> MSGGSPAEREAGRIVVRGDVAIAEAVVRKVGEVAGKEVILLISYRKNGEWITYQRNLEATP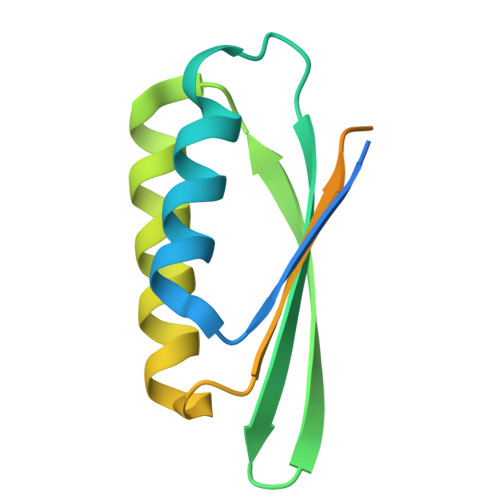EDVERTIAVIREIYEESGGDFILAIFSDPEVGAAGRAVAAAAAGGSGSHHWGSTHHHHHH> LPLTKVDSITT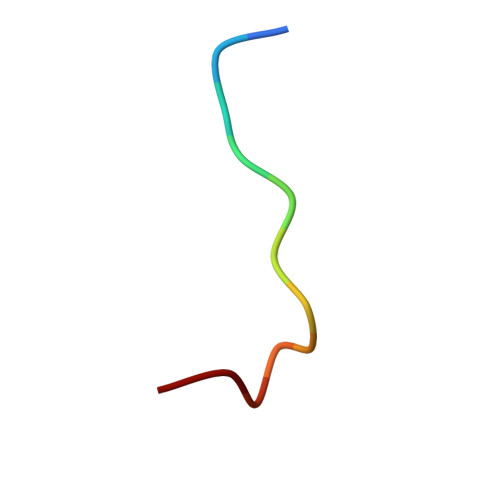F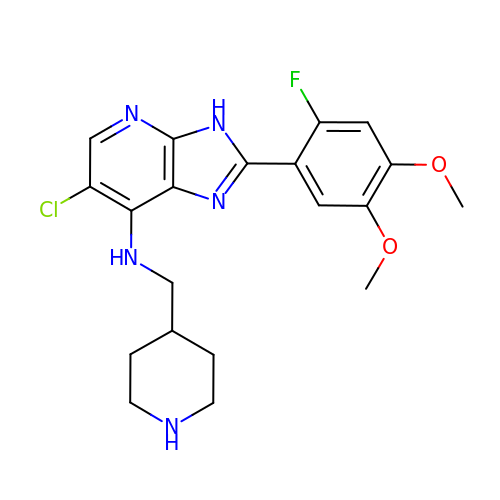6-chloro-2-(2-fluoro-4,5-dimethoxyphenyl)-N-(piperidin-4-ylmethyl)-3H-imidazo[4,5-b]pyridin-7-amine | C20 H23 Cl F N5 O2 | IRGAIDAWHGYOKD-UHFFFAOYSA-N Human NAD-IDH is a key enzyme in the TCA cycle, which catalyzes the oxidative decarboxylation of ICT into α-KG. The α and β subunits form a heterodimer (αβ), and the α and γ subunits form another heterodimer (αγ), which are assembled into a heterotetramer (α2βγ) and further into a heterooctamer (the heterotetramer and heterooctamer are also called holoenzyme). Our previous biochemical studies demonstrated that the αγ heterodimer alone exhibits a high enzymatic activity and kinetic properties comparable with those of the holoenzyme and can be activated by CIT and ADP but inhibited by NADH; on the other hand, the αβ heterodimer alone exhibits a low activity and cannot be activated by the activators but can be inhibited by NADH. Our structural comparisons show that the αβ heterodimer has a similar yet more compact overall structure compared with the αγ heterodimer and contains a pseudo-allosteric site that exhibits substantial conformational differences from the allosteric site in the αγ heterodimer.

Crystals of the αβ heterodimer with the α subunit bound with an NADH at the active site (αNADHβ) also grew at condition II with the protein solution incubated with α-KG and NADH (both 50 mm) before crystallization and belong to space group P21, and the structure was determined at 3.30 Å resolution with each asymmetric unit containing four αNADHβ molecules, which form two dimers of heterodimers via the clasp domains. In this structure, there is clear electron density for an NADH but no electron density for Ca2+ or α-KG at the active site. Unlike the αMg+NADHγNADH structure, in the αNADHβ structure, NADH binds only to the active site and occupies the spatial position of NAD. The αNADHβ structure is almost identical to the αNADβ structure (superposition of the two structures yields an RMSD of 0.5 Å for about 610 Cα atoms). The NADH binding induces almost identical conformational changes of the large domain of the α subunit as the NAD binding, and the NADH retains almost identical interactions with the surrounding residues as the NAD. These results indicate that NADH competes with NAD to bind to the active site of the αβ heterodimer and thus inhibits the activity of the αβ heterodimer. In the αNADβ and αNADHβ structures, most residues of the α and β subunits, including the β2-α2 and β3-α3 loops of the β subunit, are well-defined except a few residues at the N and C termini of the α and β subunits. On the other hand, the inactive overall conformation of the αNADβ and αNADHβ structures could be attributed to the NAD binding–induced conformational change at the active site and a newly established hydrogen-bonding network, which stabilize the side chain of Tyr-126A and the β5A-β6A loop in the inactive conformations and further trigger the conformational changes of the heterodimer interface and the pseudo-allosteric site.

>[4x]GSTGGVQTVTLIPGDGIGPEISAAVMKIFDAAKAPIQWEERNVTAIQGPGGKWMIPSEAKESMDKNKMGLKGPLKTPIAAGHPSMNLLLRKTFDLYANVRPCVSIEGYKTPYTDVNIVTIRENTEGEYSGIEHVIVDGVVQSIKLITEGASKRIAEFAFEYARNNHRSNVTAVHKANIMRMSDGLFLQKCREVAESCKDIKFNEMYLDTVCLNMVQDPSQFDVLVMPNLYGDILSDLCAGLIGGLGVTPSGNIGANGVAIFESVHGTAPDIAGKDMANPTALLLSAVMMLRHMGLFDHAARIEAACFATIKDGKSLTKDLGGNAKCSDFTEEICRRVKDLD;>ASRSQAEDVRVEGSFPVTMLPGDGVGPELMHAVKEVFKAAAVPVEFQEHHLSEVQNMASEEKLEQVLSSMKENKVAIIGKIHTPMEYKGELASYDMRLRRKLDLFANVVHVKSLPGYMTRHNNLDLVIIREQTEGEYSSLEHESARGVIECLKIVTRAKSQRIAKFAFDYATKKGRGKVTAVHKANIMKLGDGLFLQCCEEVAELYPKIKFETMIIDNCCMQLVQNPYQFDVLVMPNLYGNIIDNLAAGLVGGAGVVPGESYSAEYAVFETGARHPFAQAVGRNIANPTAMLLSASNMLRHLNLEYHSSMIADAVKKVIKVGKVRTSDMGGYATCHDFTEEICRRVKDLDENLYFQ[4x]Homoserine dehydrogenase (HSD) catalyzes NAD(P)H-dependent production of homoserine from L-aspartate-4-semialdehyde and functions in the aspartate pathway, catalyzing the synthesis of cysteine, threonine and methionine from aspartate in plants, fungi, yeast, bacteria and archaea. When overexpressed as an immature enzyme in the mesophilic bacterium Escherichia coli, recombinant homoserine dehydrogenase from the hyperthermophilic archaeon Sulfurisphaera tokodaii (StHSD) was markedly activated by heat treatment. Comparison among the structures of the immature enzyme and previously reported structures of mature enzymes revealed that a conformational change in a flexible part (residues 160–190) of the enzyme, which encloses substrates within the substrate-binding pocket, is smaller in the immature enzyme. Thus, specific conformational changes within the catalytic region appear to be responsible for heat-induced activation.

The immature enzyme was further purified using a Blue Sepharose column which is an affinity column for purification of enzymes requiring adenyl group-containing molecules, such as NAD(P)+ and ATP. Since StHSD binds to a Blue Sepharose column instead of NAD(P)+, the enzyme in the eluant after binding to the column should be the apo-form. The absence of NAD(P)+ from the purified enzyme was also confirmed by structural analysis of the immature enzyme. The structure of the immature apoenzyme was designated the IM structure. In the immature apoenzyme, the substrate-binding pocket assumes a more closed form than in the mature apoenzyme. Upon NAD(P)+ binding, the lid part interacts with the rigid part and changes its location substantially to form a hydrogen bond between E186 and R38. The distance between the rigid and lid parts within the IM structure (cyan in Fig. 6c) is larger than within the M structure (represented in pink in Fig. 6c). Heat treatment-induced conformational changes were more obvious in a region of residues 181–190 in the apo-form than those observed in the substrate analog-bound forms. All the structures obtained here had a disulfide bond between the C303 residues in the C-terminal regions of the two subunits. The distance between the two sulfur atoms in both the IM and IM/NADP/BU structures was 2.1 Å, which is similar to that in the oxidized enzyme (the M structure; 2.2 Å) but less than that in the reduced enzyme (2.9 Å).

>[2x]MKLLLFGYGNVGKAFRKLLHEKRSPELNDVIIGGIVTRRGIMLQDKEDFTPDLEGDVFKAFEKIKPDIIVDVSSANYNNGEPSLSLYKEAIKDGVNIITTNKAPLALAFNEIFSLARSKGVKIGFQGTVMSGTPSINLYRVLPGSRVIKIRGILNGTTNFILTLMNKGVSFEEALKEAQRRGYAEEDPTLDINGFDAAAKITILANFMIGNSVTIKDVKFEGINRDLPKNEKIKLIAYADEKEVWVKPLPISQDDPLYNVDGVENALEITTDIQSILIRGPGAGPVNAAYGALSDLILLKRDCL>[4x]SALKEIQEAYILSGARTPTAKFNGSFVSVSAPELGAVAIKSAVSKSGVPVEKITDVYMGNVLQGAVGQAPARQASMFAGLSPTVESMTVNKVCASGLKAVALAAQNIQLGLAEAQVAGGMENMSRVPYYLPRSTQLPPFGEIKLQDGLIQDGLWDVYNQFHMGICAEKTAKKYEISREEQDQYAIQSYQRAQAAWKENKFAEEIAPVTVKGKKGETVVERDEGYENLRIDKMATLKPAFLRDGTGTVTAGNASTMNDGASALVLGSKAIAREFAQGNRALARIVSTADAAIDPVDFPVAPAKAVPIALERAGITKDQVAVWEFNEAFAAVIKANEKILGLQNARVNPLGGAISLGHALGSSGSRILVTLLHQLQPGEYGVAAICNGGGAATAMVVQKLDRVD

In this study, we have characterized recombinant AfERG10A as a functional acetyl-CoA acetyltransferase catalyzing both synthetic and degradative reactions. Unexpectedly, AfERG10A localizes to the mitochondria in A. fumigatus, as shown by C-terminal green fluorescent protein (GFP) tag fusion. Both knockout and inducible promoter strategies demonstrate that Aferg10A is essential for the survival of A. fumigatus. AfERG10A consists of three domains, an N-terminal domain (residues Glu36 to Asn153 and Asn287 to Arg302), a C-terminal domain (residues Ala312 to Asp433), and a loop domain (residues Met154 to Met286).

To provide insight into the structural prerequisites and find potential exploitable differences between AfERG10A and human orthologues, structures of apo- and CoA-complexed AfERG10A were determined using crystals grown from conditions of 0.1 M HEPES (pH 7.0) and 2 M ammonium sulfate in the absence or presence of CoA. In one asymmetric unit, there are four molecules (A to D) forming a tetramer, which is similar to other members of thiolase family, such as in humans, S. cerevisiae, and E. coli. By comparison, the root mean square deviation (RMSD) value between the apo- and CoA-bound structures is 0.175 Å, with 367 atoms matched, suggesting that CoA binding does not cause major conformation change. Although the catalytic machinery of AfERG10A and human ACATs is fully conserved, a close inspection of the CoA binding site revealed exploitable differences. For instance, residues binding to adenosine 3′-phosphate of CoA are Asn257, Leu258, and Arg259 in AfERG10A, whereas they are Arg258, Val259, and Asp260 in ACAT1 and Gly225, Ser226, and Asn227 in ACAT2. Met286 in AfERG10A binding to the pantetheine moieties of the CoA molecule is equivalent to Leu286 in ACAT1 and Ile254 in ACAT2. Those differences reveal that AfERG10A possesses potentially exploitable differences in the CoA binding site compared to the human orthologues. Encouragingly, by solving the crystal structure of AfERG10A and superimposing it with structures of human orthologues, four different residues within the CoA binding site were discovered. This will be the structural basis for a rational design of specific antifungal inhibitors targeting AfERG10A.> GP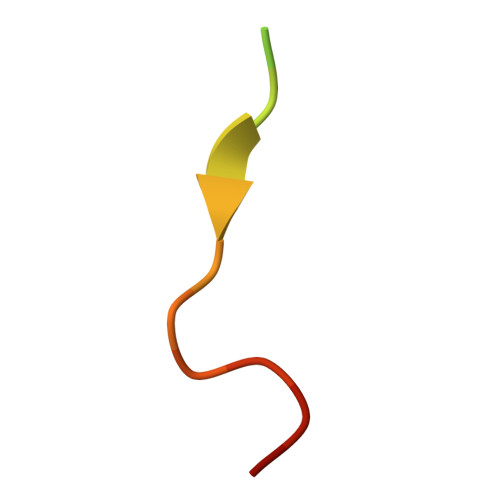LGSPADTCIYNPLFGSD>MFKTEFEFPEELKTKLQEHINYFPKKRQAILLCLHEIQNYYGYIPPESLKPLADMLELPLNHVEGVVAFYDMFDREDKAKYRIRVCVSIVCHLMGTNKLLKALENILGIKPGEVTPDGKFKIVPVQCLGACSEAPVFMVNDDEYKFESEVQLNEILSRYT[2x];>MRSYPAIPRIYAETTLNMLLKRAKKPRVHSIDEYLKDGGYQALEKALNMSPEEIIDWVDKSTLRGRGGAGFPTGKKWKFAVQNPGPRYFICNADESEPGTFKDRIIIERDPHLLIEGIIISSYAIGANEAYIYIRGEYPAGYYILRDAIEEAKKKGFLGKNILGSGFDLEIYVARGAGAYICGEETALIESLEGKRGHPRLKPPYPVQKGLWGKPTVVNN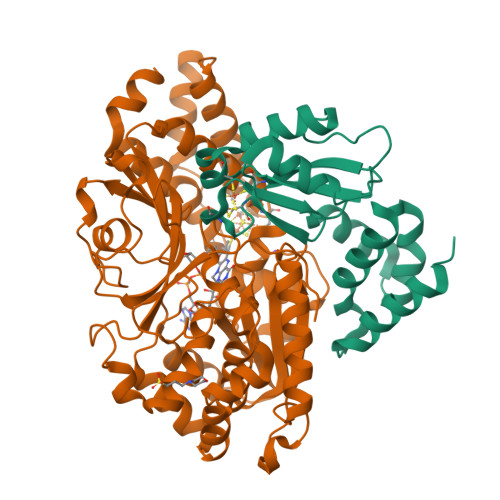VETIANVPFIISMGWEEYRYIGPSDYAGPKLFPVSGKVKKPGVYELPMNTTLREVIFKYAGGTLGNKKVKAVFSGALDCFSSEELDIPMDYSPLGFGGTGTVIVLTEEDDIVEAALKIAEFYEHETCGQCTPCRVGCYEQANLLEKIYKGEATEQDWEGFDFVNRNIQPTSICGLGAVAGRLIRQTLEKFPEEWEKYRKKSASLPLAGHHHHHH[2x]2-chloro-4-{(2-methylbenzyl)[(3S)-1-(methylsulfonyl)pyrrolidin-3-yl]amino}benzonitrile | C20 H22 Cl N3 O2 S | 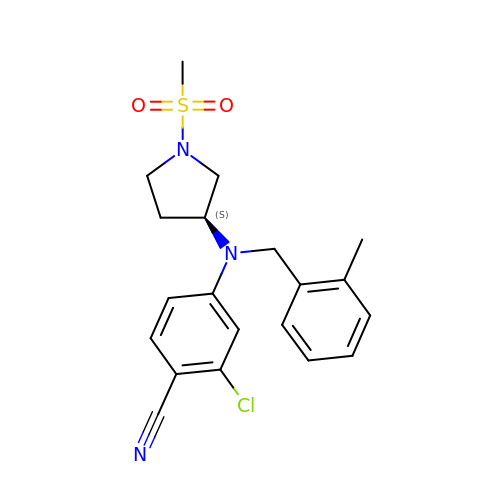OTRAFCFYTZJLKH-IBGZPJMESA-N> PIFLNVLEAIEPGVVCAGHDNNQPDSFAALLSSLNELGERQLVHVVKWAKALPGFRNLHVDDQMAVIQYS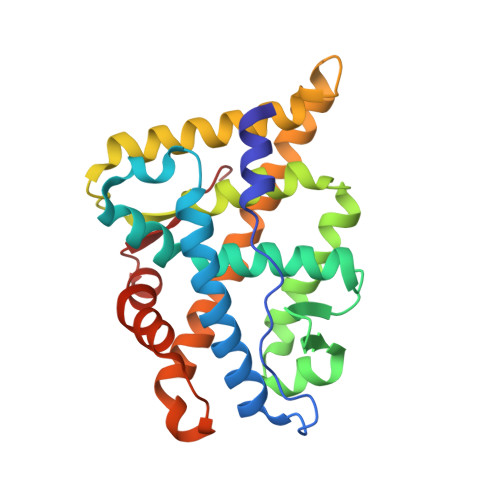WMGLMVFAMGWRSFTNVNSRMLYFAPDLVFNEYRMHKSRMYSQCVRMRHLSQEFGWLQITPQEFLCMKALLLFSIIPVDGLKNQKFFDELRMNYIKELDRIIACKRKNPTSCSRRFYQLTKLLDSVQPIARELHQFTFDLLIKSHMVSVDFPEMMAEIISVQVPKILSGKVKPIYFHT4-{(2S, 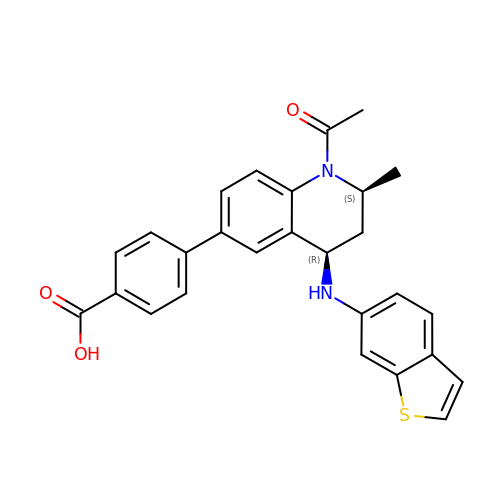4R)-1-acetyl-4-[(1-benzothiophen-6-yl)amino]-2-methyl-1,2,3,4-tetrahydroquinolin-6-yl}benzoic acid | C27 H24 N2 O3 S | PSXHCEJOKMTHEO-UPCLLVRISA-N> GQLAPGITMSEIDRIAQNIIKSHLETCQYTMEELHQLAWQTHTYEEIKAYQSKSREALWQQCAIQITHAIQYVVEFAKRITGFMELCQNDQILLLKSGCLEVVLVRMCRAFNPLNNTVLFEGKYGGMQMFKALGSDDLVNEAFDFAKNLCSLQLTEEEIALFSSAVLISPDRAWLLEPRKVQK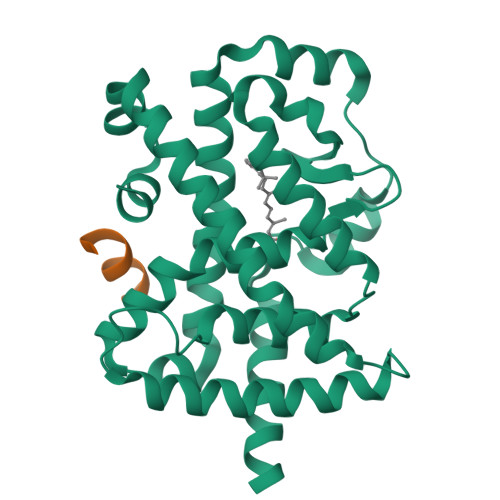LQEKIYFALQHVIQKNHLDDETLAKLIAKIPTITAVCNLHGEKLQVFKQSHPDIVNTLFPPLYKELFNPDCAAVCK;> RHKILHRLLQEGSPS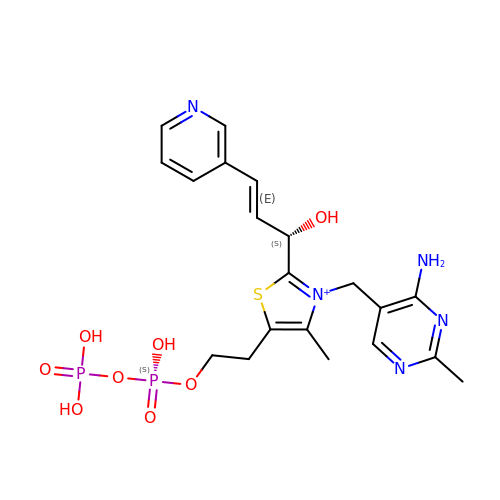3-[(4-amino-2-methylpyrimidin-5-yl)methyl]-5-(2-{[(S)-hydroxy(phosphonooxy)phosphoryl]oxy}ethyl)-2-[(1S,2E)-1-hydroxy-3-pyridin-3-ylprop-2-en-1-yl]-4-methyl-1,3-thiazol-3-ium | C20 H26 N5 O8 P2 S | HUCLASQGRJZNFE-RTRPANQVSA-O>[2x]GGACUCGGGGUGCCCUUCUGCGUGAAGGCUGAGAAAUACCCGUAUCACCUGAUCUG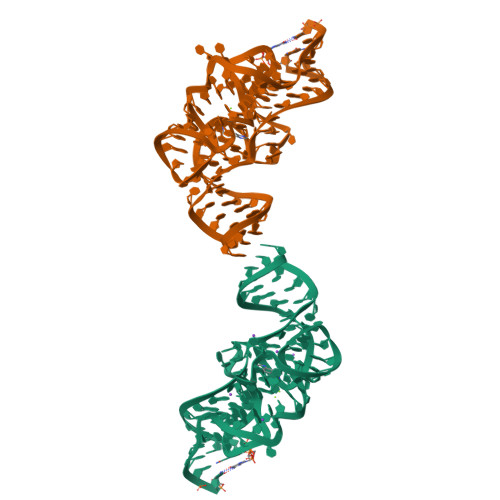GAUAAUGCCAGCGUAGGGAAGUUC> MQRSTAVVDGSQQVDPAMLAALQSQPSGVTPSDDWAAAMDRILALTTRNPEAFRQQPQANRFSAILEAVVPSRTNPTHEK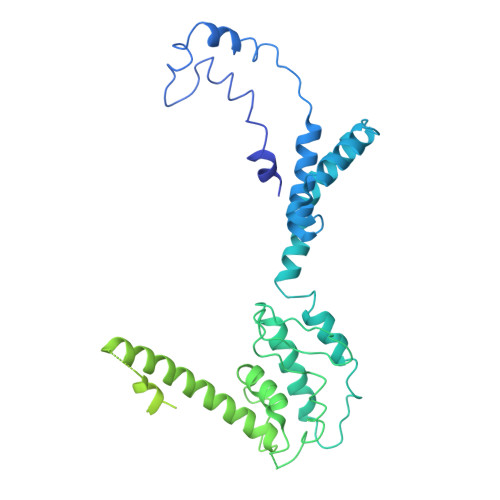VLAIVNALTESKAIRKDEAGLIYNALLERVARYNSTNVQANLDRLTTDVREAVAQRERFMHDTNLGSQVALNAFLSTLPANVPRGQEDYVSFISALRLLVAEVPQSEVYQSGPDYFFQTSRQGLQTVNLTQAFKNLQGMWGVRAPVGDRATISSLLTPNTRLLLLLIAPFTNSSTISRDSYLGHLITLYREAIGQTQVDEQTFQEITSVSRALGQQDTGSLEATLNFLLTNRQQKIPSQFTLSTEEERILRYVQQSVSLYLMREGMTPSSALDMTARNMEPSLYSSNRPFINRLMDYLHRAAAMNSEYFTNAILNPHWMPPSGFYTGEFDMPEGDDGFLWDDVSDSIFVPARYRKKEGGDELPLPLVEAASRGQSPFPSLPSLVSSSNSGRVLRPRLPGETDYLNDPLLQPVRNKNFPNNGVESLVDKMNRWKTYAQEQREWEESQSRPLAGPFSRWRRREDDQDDSADDNSVLDLGGTGASSNPFAHLRPQGRLGRLY>GSMDPSGVKVLETAEDIQERRQQVLDRYHRFKELSTLRRQKLEDSYRFQFFQRDAEELEKWIQEKLQIASDENYKDPTNLQGKLQKHQAFEAEVQANSGAIVKLDETGNLMISEGHFASETIRTRLMELHRQWELL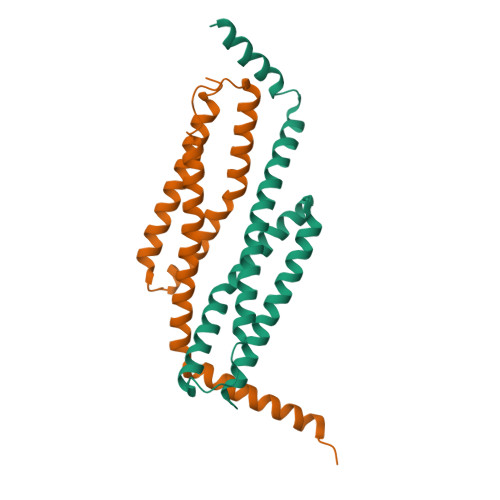LEKMREKGIKLLQ[2x]3-cyano-N-(3-{[(3S)-4-(cyclopentanecarbonyl)-3-methylpiperazin-1-yl]methyl}-5-fluoro-2-methylphenyl)benzamide | C27 H31 F N4 O2 | 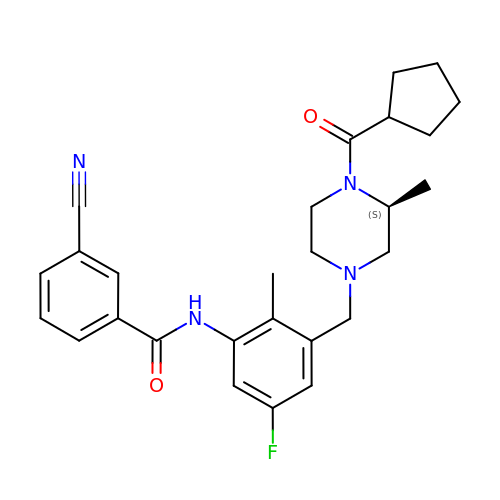AQGBWBMWWNRWNU-SFHVURJKSA-N6-cyclobutyloxy-9-ethyl-~{N}-[(4-ethylsulfonylphenyl)methyl]carbazole-3-carboxamide 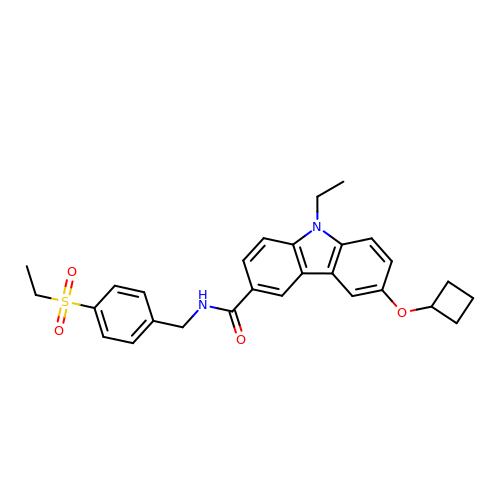| C28 H30 N2 O4 S | LWRIAGPHTVDVJI-UHFFFAOYSA-N> MADSDLPTKGRQRGVRAVELNVAARLENLALLRTLVGA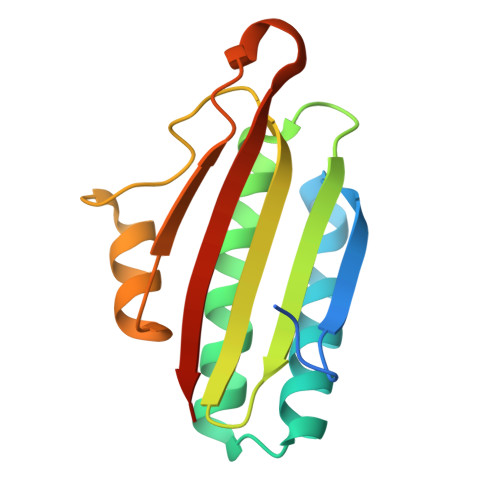IGTFEDLDFDAVADLRLAVDEVCTRLIRSALPDATLRLVVDPRKDEVVVEASAACDTHDVVAPGSFSWHVLTALADDVQTFHDGRQPDVAGSVFGITLTARRAASSR>[12x]MQLFDLSLEELKKYKPKKTARPDFADFWKKSLEELRQVEAEPTLESYDYPVKGVKVYRLTYQSFGHSKIEGFYAVPDQTGPHPALVRFHGYNASYDDGIHDIVNWALHGYATFGMLVRGQGGSEDTSVTPGGHALGWMTK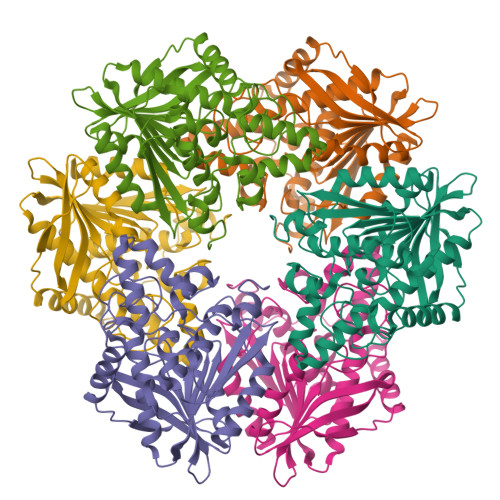GILSKDTYYYRGVYLDAVRALEVIQSFPEVDEHRIGVIGGSQGGALAIAAAALSDIPKVVVADYPYLSNFERAVDVALEQPYLEINSYFRRNSDPEVEEKAFETLSYFDLINLAGWVKQPTLMAIGLIDQVTPPSTVFAAYNHLETDKELKVYRYFGHEFIPAFQTEKLSFLQKHLLLST Autophagy-related protein 18 (Atg18) participates in the elongation of early autophagosomal structures in concert with Atg2 and Atg9 complexes. Atg18 belongs to the protein family of β-propellers that bind polyphosphoinositides (PROPPIN). The corresponding primary structure contains a series of conserved WD40 repeats forming the 6 or 7 blades of a β-propeller fold. The autophagic membrane adapter Atg18 reveals an unexpected structural plasticity in multiple modes of oligomeric organization.

In an effort to improve the helical order, we imaged the previously characterized Atg18-P72A/R73A (PR72AA) mutant that has lost its ability to interact with Atg241. The corresponding Fourier transforms supported the same structural organization of both helical assemblies, with an improved helical ordering in the Atg18-PR72AA mutant over the Atg18-WT, indicated by the higher diffracting layer line at 1/6 Å. D Fourier shell correlation threshold at 0.143 indicates resolutions of 3.8 and 3.3 Å for the 3D structures of Atg18-WT and Atg18-PR72AA, respectively. The helical symmetry unit is illustrated with alternating blue/white colors (pitch: 100 Å, number of units per turn 5.1; helical rise: 19.4 Å, rotation 70.0°). The T-interface includes R285 and R286 of the FRRG motif that are in direct contact with blade 6 of the adjacent molecule. The I-interface is located between blade 3 and blade 4 due to a 180° disc rotation a pseudo dihedral symmetry including in a small tilt of the two discs with respect to each other. Notably, four T-interfaces are arranged in the characteristic lozenge pattern that was previously observed in the COPII coat formed by Sec31 tetramers. In fact, the T-interface buries the PI3P/PI(3,5)P2 FRRG binding interface and shows direct competition between PIP binding and tube formation. Similarly, Atg18 phosphorylations in loop 7AB can be expected to affect the stability of the tubular assembly, in particular, as the higher resolution structure of Atg2-binding deficient mutant Atg18-PR72AA tubes suggested an increased rigidity over Atg18-WT.

>MSDSSPTINFINFNQTGTCISLGTSKGFKIFNCEPFGKFYSEDSGGYAIVEMLFSTSLLALVGIGDQPALSAARLRIINTKKHSIICEVTFPTSILSVKMNKSRLVVLLQEQIYIYDINTMRLLHTIETNPNPRGLMAMSPSVANSYLVYPSPPKVINSEIKAHATTNNITLSVGGNTETSFKRDQQDAGHSDISDLDQYSSFTKRDDADPTSSNGGNSSIIKNGDVIVFNLETLQPTMVIEAHKGEIAAMAISFDGTLMATASDKGTIIRVFDIETGDKIYQFRRGTYATRIYSISFSEDSQYLAVTGSSKTVHIFKLGHSMSNNKLDSDDSNMEEAAADDSSLDTTSIDALSDEENPTRLAREPYVDASRKTMGRMIRYSSQKLSRRAARTLGQIFPIKVTSLLESSRHFASLKLPVETNSHVMTISSIGSPIDIDTSEYPELFETGNSASTESYHEPVMKMVPIRVVSSDGYLYNFVMDPERGGDCLILSQYSILMD[4x]>[2x]AQKSVKISDDISITQLSDKVYTYVSLAEIEGWGMVPSNGMIVINNHQAALLDTPINDAQTEMLVNWVTDSLHAKVTTFIPNHWHGDCIGGLGYLQRKGVQSYANQM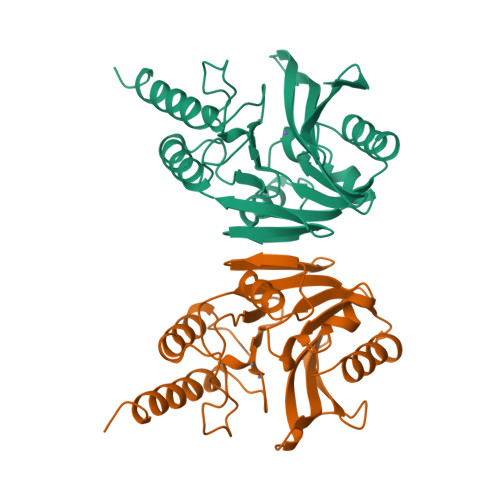TIDLAKEKGLPVPEHGFTDSLTVSLDGMPLQCYYLGGGHATDNIVVWLPTENILFGGCMLKDNQATSIGNISDADVTAWPKTLDKVKAKFPSARYVVPGHGDYGGTELIEHTKQIVNQYIESTSKP>SNAMLQKINRYTHGFVAVPVILACREKGVFELLADESPLSLNQMVEHLGANSGHFQVALRMLESLHWLSRNKELKYSLTAEAAIHNKISEDILQLYNLPIQSYLEGKQGNLLGRWIERSCQLWNLDNPLMADFLDGLLVIPLLLALHKHNLLADSEDKPLLSSLSSTVQEELGKLFLHLGWADLTAGRLTITELGRFMGERALNTAIVASYTPMLSRIHDVLFGNCLS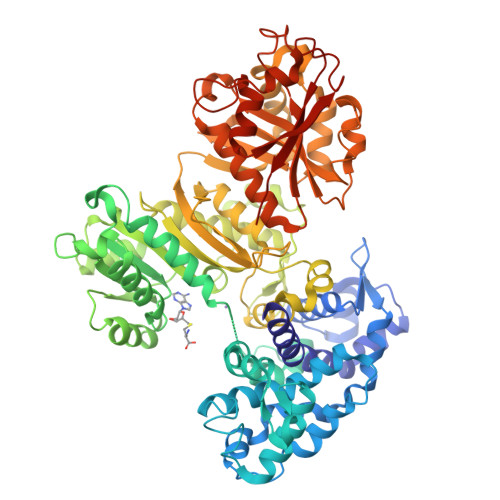VFQRDASGHERHIDRTLNVIGSGFQHQKYFADLEESILSVFNQLPLEEQPKYITDMGCGDGTLLKRVWETIQFKSARGKALEQYPLRLIGVDYNEASLKATTRTLASLPHLVLQGDIGNPEQMVRSLEAHGIHDPENILHIRSFLDHDRLFIPPQKRNELKERAHLPYQSVCVDDQGELIPPHVMVQSLVEHLERWSQVVNKHGLMILEVHCLEPRVVYQFLDKSENLHFDAFQGFSQQYLVEAEVFLMSAAQVGLFPKLELSKRYPKTFPFTRITLNYFEKRPYKISHAYLSDLPALVDLEVKCWPENLRASTHEIRRRLELNPQGNLVLIIEDQIIGAIYSQTITSTEALENVKYAQVPTLHTPQGSVIQLLALNILPEFQARGLGNELRDFMLYYCTLKGGIESVVGVTRCRNYVNYSQMPMMEYLKLHNEQRQLLDPIVGFHVSGGAEIRGIIANYRPEDTDNLGMGILIEYNLRDSALHS[2x]>GSGPLKPE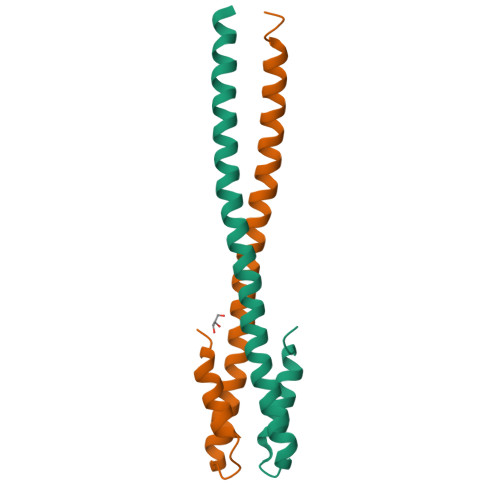EHEDILNKLLDPELAQSERTEALQQLRVNYGSFVSEYNDLTKDYTRVNDDVAAQQATNAKLKARNDQLFAEIDDLNGG[4x]>MILIADSGSTKTHWNVLDQGRVIGEIFTKGMNPFFQTPEEMGREIERTLLPQLNSNRFCEVHFFGAGCIPEKVPVVRNVLKGCLDVSSLIEVDTDMLAAAKASCGRSPGIVCIMGTGSNSCFYDGEKIAANVSPLGFILGDEGSGAVLGKLLIGDLLKNQMGEELKEKFLRQYELTPANIIERVYRQPFPNRFLAGISPFLAENIEHPAIHSLVLNAFKSFLTRNVMQFDYTRYKAHFIGSVAYYYKDILEEAAAATGIRTGTI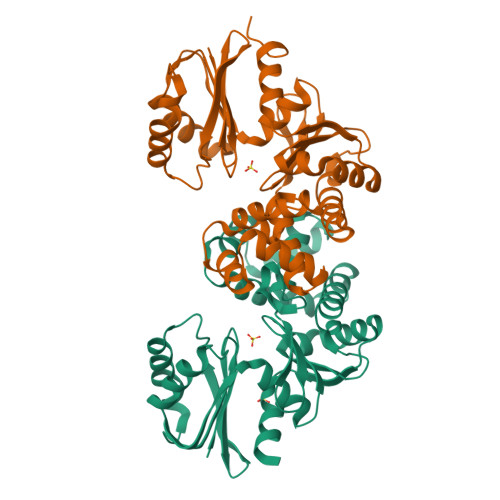VRNPMEGLRTYYSTVAKTV[4x]> GAMDPEFNPFNVELISSLLESIDFSMY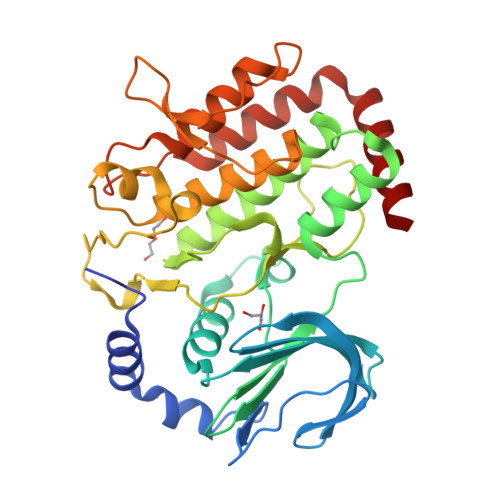IEKLPHCQLVGHVKRLHPNTHLEVHNEKFEVSKMIGKGAYGSVYVGKHLKSGKKVALKQERPTNYWEFYICLEIHSRLTSEQMIPSYAHIDYALVGNNSSVYISEFSDYGSLIGVCNKVKSVTNRNMDEYVVMHLSCQMLDIVDHLHAMGIIHADIKPDNFLLMKPICADPNEVSLQLIDFGVSIDMKLFPDNQTFNYVHHDDLFKCIEMRTGRPWTYQLDLYGLVSVMHVLLFGRYMEVVQRSPSTIWMPKTNVPRYFQRTMWENIFRTLLNIRDCRTMPNLQQLRTQLKCALAEKEKYVAEAISKFNTILQK>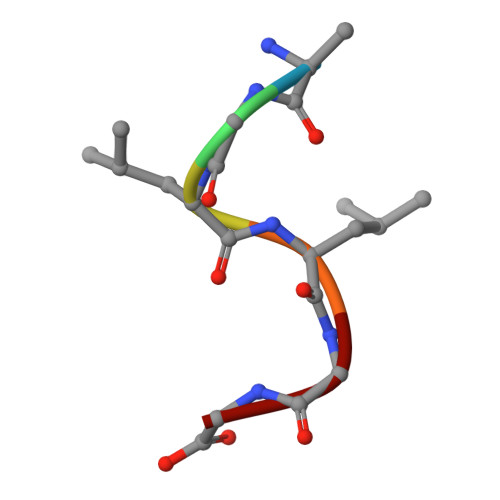 IGLLGG>[8x]ESQPDPKPDELHKSSKFTGLMENMKVLYDDNHVSAINVKSIDQFLYFDLIYSIKDTKLGNYDNVRVEFKNKDLADKYKDKYVDVFGANYYYQCYFSKKTNDINSHQTDKRKTCMYGGVTEHNGNQLDKYRSITVRVFEDGKNLLSFDVQTNKKKVTAQELDYLTRHYLVKNKKLYEFNNSPYETGYIKFIENENSFWYDMMPAPGDKFDQSKYLMMYNDNKMVDSKDVKIEVY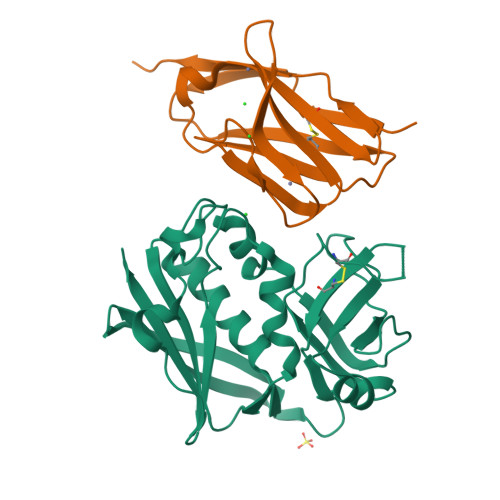LTTKKK;>[8x]MARLEAAVTQSPRNKVAVTGEKVTLSCKQTNSYFNNMYWYRQDTGHELRLIFMSHGIRNVEKGDIPDGYKASRPSQENFSLILELATPSQTSVYFCASGGGGTLYFGAGTRLSVLYGSSRVDLQP> MIHQNTIYTAGIETEEQVSQLTERISNMIGVHQVNINIIDGQVTV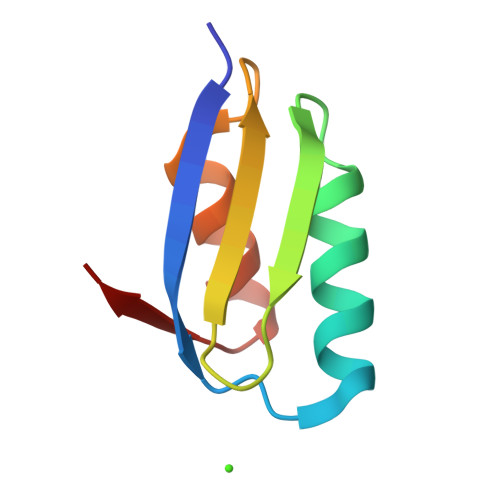SYETPANLNSIEKEIYDEGYKIVF> GQDRSEATLIKRFKGEGVRYKAKLIGIDEVSAARGDKLCQDSMMKLKGVVAGARSKGEHKQKIFLTISFGGIKIFDEKTGALQHHHAVHEISYIAKDITDHRAFGYVCGKEGNHRFVAIKTAQAAEPVILDLRDLFQLIYELKQREELEKKA;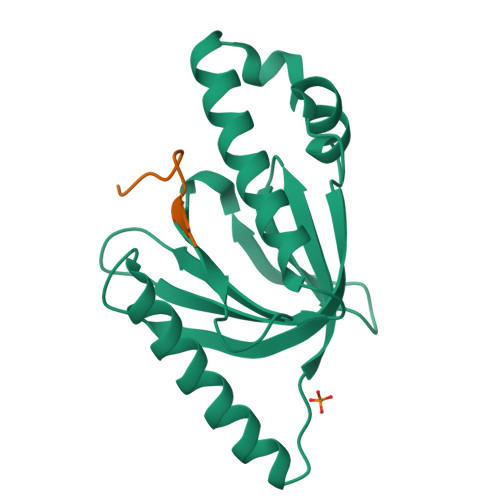> NFDNPVYRKT>[2x]MDMLWHKLPKSIYFRRGSLPIALDEVITDGHKRALIVTDRFLFNNGYADQITSVLKAAGVETEVFFEVEADPTLSIVRKGAELANSFKPDVIIALGGGSPMDAAKIMWVMYEHPETHFEELALRFMDIRKRIYKFPKMGVKAKMIAVTTTSGTGSEVTPFAVVTDDATGQKYPLADYALTPDMAIVDANLVMDMPKSLCAFGGLDAVTHAMEAYVSVLASEFSDGQALQALKLLKEYLPASYHEGSKNPVARERVHSAATIAGIAFANAFLGVCHSMAHKLGSQFHIPHGLANALLICNVIRYNANDNPTKQTAFSQYDRPQARRRYAEIADHLGLSAPGDRTAAKIEKLLAWLETLKAELGIPKSIREAGVQEADFLANVDKLSEDAFDDQCTGANPRYPLISELKQILLDTYYGRDYVEGETAAKKEAAPAKAEKKAKKSAPWGAGGLEVLFQ

The bifunctional alcohol/aldehyde dehydrogenase (AdhE) comprises both an N-terminal aldehyde dehydrogenase (AldDH) and a C-terminal alcohol dehydrogenase (ADH). AdhE is a crucial enzyme primarily in alcohol metabolism and catalyzes the conversion of the high-energy substrate acetyl-CoA to acetaldehyde and subsequently to ethanol. In vivo, full-length AdhE oligomerizes into long oligomers known as spirosomes. As has been shown previously, the alcohol dehydrogenase domain of AdhE forms homodimers that are essential for the formation of the larger full-length AdhE spirosomes.

Here, we describe the atomic structure of the cofactor-bound ADH domain from E. coli determined by X-ray crystallo­graphy to 1.65 Å resolution. The two forms superimpose well, with a root-mean-square deviation (r.m.s.d.) of 0.32 Å over 404 Cα atoms, and interestingly there are no obvious local differences in the binding site for NAD. The benzamide part of the NAD molecule is less ordered in the electron density, and it is likely that this part does not form strong interactions with ADH, allowing the moiety to exhibit a number of conformations. This is reflected in the B factors of the NAD moiety, where the adenosine diphosphate has an average B factor of 26 Å2 and the ribose-benzamide end has an average B factor of 49 Å2, which is higher than the average B factor of the protein model of 28 Å2. NAD interactions correspond to 3% of the total accessible surface area of ADH. Additional electron density was observed in the metal ion-binding site, as previously found in gADH, where it was identified as Zn2+. As ADH has been described as being reliant on binding to iron this density has been modelled as Fe2+, although it may also be a Zn2+ ion as observed in the homologue from G. thermoglucosidasius. The metal ion is coordinated by Asp653, His657, His723 and His737 with additional waters.> KCPQPKTLDEFTIIQNLQPQYQFRDYFIATCKQGYQLIEGNQVLHSFTAVCQDDGTWHRAMPRCKIKDCGQPRNLPNGDFRYTTTMGVNTYKARIQYYCHEPYYKMQTRAGSRESEQGVYTCTAQGIWKNEQKGEKIPRCLPVCGKPVNPVEQRQRIIGGQKAKMGNFPWQVFTNIHGRGGGALLGDRWILTAAHTLYPKEHEAQSNASLDVFLGHTNVEELMKLGNHPIRRVSVHPDYRQDESYNFEGDIALLELENSVTLGPNLLPICLPDNDTFYDLGLMGYVSGFG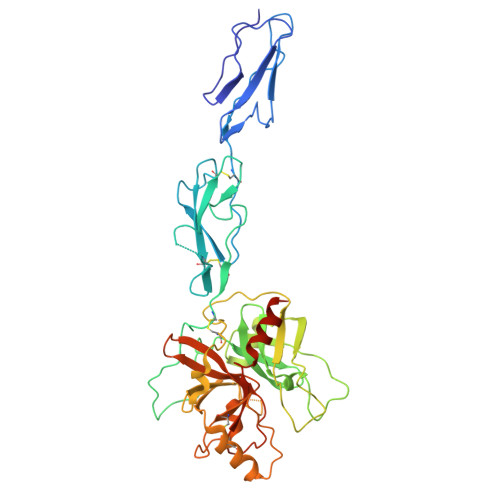VMEEKIAHDLRFVRLPVANPQACENWLRGKNRMDVFSQNMFCAGHPSLKQDACQGDAGGVFAVRDPNTDRWVATGIVSWGIGCSRGYGFYTKVLNYVDWIKKEMEEEDGSGHHHHHHHH>MGSSHHHHHHGSIDFSNAPKRLNNKYPLSDQKNEGGWVLNKKASDEFKGKKLNEERWFPNNPKWKGRQPTFFAKENTTFEDGCCVMRTYKPEAGSLPEGYTHTAGFLVSKELFLYGYFEARLRPNDSPWVFGFWMSNNERNWWTEIDICENCPGNPANRHDLNSNVHVFKAPADKGDIKKHINFPAKYYIPFELQKDFHVWGLDWSKEYIRLYIDGVLYREIENKYWHQPLRINLNNESNKWFGALPDDNNMDSEYLID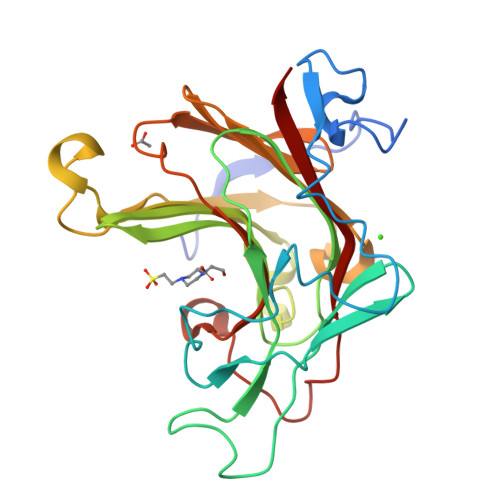YVRVWYKK[3x]>[4x]AQQNILSVHILNQQT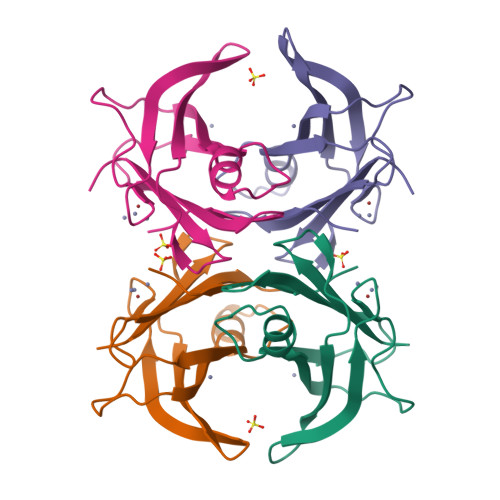GKPAADVTVTLEKKADNGWLQLNTAKTDKDGRIKALWPEQTATTGDYRVVFKTGDYFKKQNLESFFPEIPVEFHINKVNEHYHVPLLLSQYGYSTYRGS Bromodomains (BRDs) are protein interaction modules that specifically recognize ε-N-lysine acetylation motifs, a key event in the reading process of epigenetic marks. The 61 BRDs in the human genome cluster into eight families based on structure/sequence similarity. Despite large sequence variations, all BRD modules share a conserved fold that comprises a left-handed bundle of four α helices (αZ, αA, αB, αC), linked by loop regions of variable length (ZA and BC loops), which line the Kac binding site and determine binding specificity. The four helices form a deep cavity that is extended by the two loop regions (ZA and BC loops), creating a largely hydrophobic Kac binding pocket.

The C and N termini are highly diverse and may comprise additional helices that extend the canonical BRD fold (e.g., the sixth BRD of PB1 has an additional C-terminal helix) or largely extended kinked helices that are present as C- or N-terminal extensions (for instance in TAF1L or ATAD2).

> SMQEEDTFRELRIFLRNVTHRLAIDKRFRVFTKPVDPDEVPDYVTVIKQPMDLSSVISKIDLHKYLTVKDYLRDIDLICSNALEYNPDRDPGDRLIRHRACALRDTAYAIIKEELDEDFEQLCEEIQESR>GHMNLCYIDGKFLPLEEAKLPVTDLIIQRGVGVFETISTHSRRPLMLTPHLKRLEGSATASSIVMPATLDEMARIIREGIKKMGCETMVRPYITGGDSFGKDHLFSSSRYFVIFAEIRKPDPILYEKGVALHPINAERYLPSTKSINYMLSFTGQRDSKGAYEILYCPEGEIVEGSHSTFFLIKNGHLITAPTSRALSGTTRQIVLELARRGNIQVEERC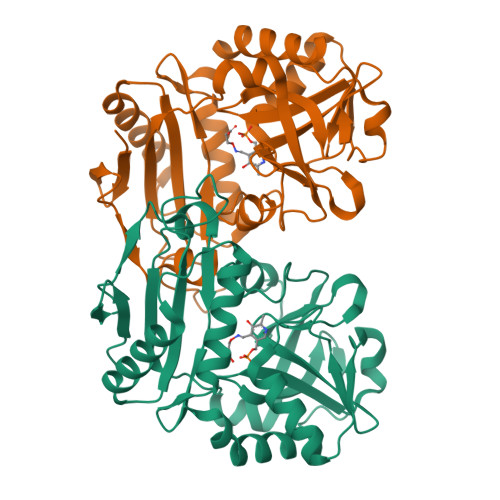PLLTELPEAEEAFITGTVKELLPVVRIGDQIIGNGVPGKLTKHLHQVYLSSIVEWLE[5x]>[4x]SNAMNDIVASTQLPNTIKTITNDLRKLGLKKGMTVIVHSSLSSIGWISGGAVAVVEALMEVITEEGTIIMPTQSSDLSDPKHWSRPPVPEEWWQIIRDNVPAFEPHITPTRAMGKVVECFRTYPNVVRSNHPLGSFAAWGRHAE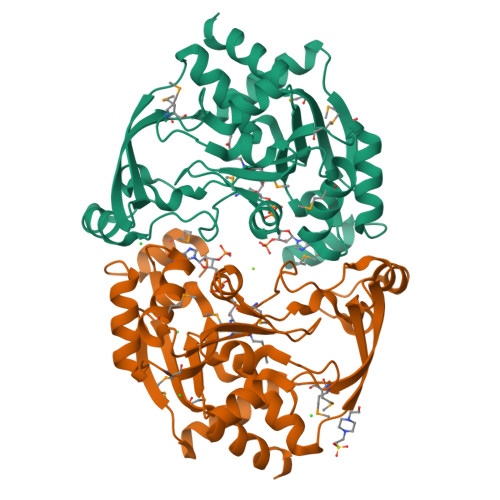EITVNQSLSMSLGEESPLRKIYDLDGYILLIGVGYDSNTSVGLSEVRSGACELIKVGAPIIENGERVWKEFVDMDYDSDKFVEIGVEFEQKGTVTMGKIGNAKCRLMKQRDIVDFGTEWFRKKN> LTLGNTTSSVILTNYMDTQYYGEIGIGTPPQTFKVVFDTGSSNVWVPSSKCSRLYTACVYHKLFDASDSSSYKHNGTELTLRYSTGTVSGFLSQDIITVGGITVTQMFGEVTEMPALPFMLAEFDGVVGMGFIEQAIGRVTPIFDNIISQGVLKEDVFSFYYNRDSENSQS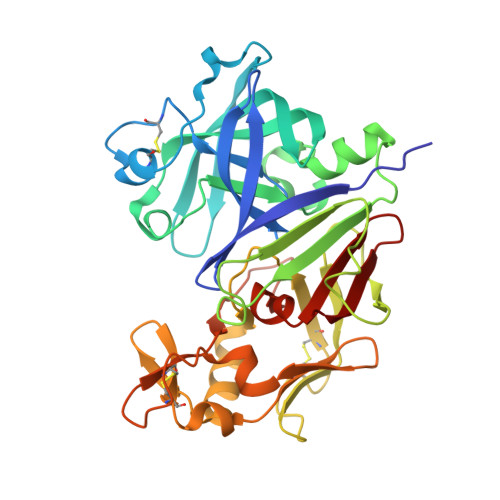LGGQIVLGGSDPQHYEGNFHYINLIKTGVWQIQMKGVSVGSSTLLCEDGCLALVATGASYISGSTSSIEKLMEALGAKKRLFDYVVKCNEGPTLPDISFHLGGKEYTLTSADYVFQESYSSKKLCTLAIHAMDIPPPTGPTWALGATFIRKFYTEFDRRNNRIGFALAR(2S)-4-(2,5-DIFLUOROPHENYL)-N-METHYL-2-PHENYL-N-PIPERIDIN-4-YL-2,5-DIHYDRO-1H-PYRROLE-1-CARBOXAMIDE 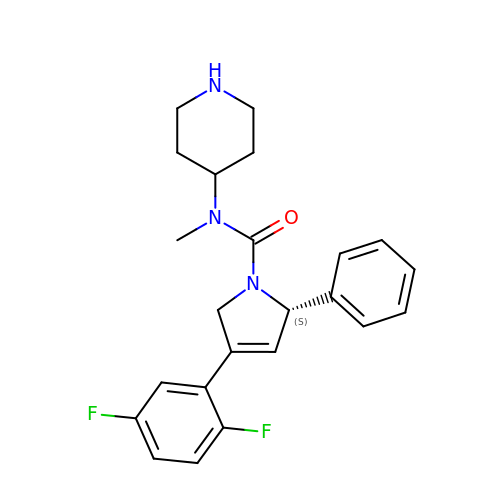| C23 H25 F2 N3 O | NKLVBHMAIMEVEH-QFIPXVFZSA-N>MSPITREERLERRIQDLYANDPQFAAAKPATAITAAIERPGLPLPQIIETVMTGYADRPALAQRSVEFVTDAGTGHTTLRLLPHFETISYGELWDRISALADVLSTEQTVKPGDRVCLLGFNSVDYATIDMTLARLGAVAVPLQTSAAITQLQPIVAETQPTMIAASVDALADATELALSGQTATRVLVFDHHRQVDAHRAAVESARERLAGSAVVETLAEAIARGDVPRGASAGSAPGTDVSDDSLALLIYTSGSTGAPKGAMYPRRNVATFWRKRTWFEGGYEPSITLNFMPMSHVMGRQILYGTLCNGGTAYFVAKSDLSTLFEDLALVRPTELTFVPRVWDMVFDEFQSEVDRRLVDGADR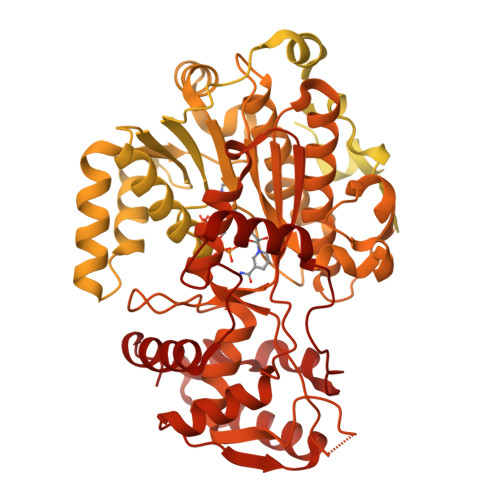VALEAQVKAEIRNDVLGGRYTSALTGSAPISDEMKAWVEELLDMHLVEGYGSTEAGMILIDGAIRRPAVLDYKLVDVPDLGYFLTDRPHPRGELLVKTDSLFPGYYQRAEVTADVFDADGFYRTGDIMAEVGPEQFVYLDRRNNVLKLSQGEFVTVSKLEAVFGDSPLVRQIYIYGNSARAYLLAVIVPTQEALDAVPVEELKARLGDSLQEVAKAAGLQSYEIPRDFIIETTPWTLENGLLTGIRKLARPQLKKHYGELLEQIYTDLAHGQADELRSLRQSGADAPVLVTVCRAAAALLGGSASDVQPDAHFTDLGGDSLSALSFTNLLHEIFDIEVPVGVIVSPANDLQALADYVEAARKPGSSRPTFASVHGASNGQVTEVHAGDLSLDKFIDAATLAEAPRLPAANTQVRTVLLTGATGFLGRYLALEWLERMDLVDGKLICLVRAKSDTEARARLDKTFDSGDPELLAHYRALAGDHLEVLAGDKGEADLGLDRQTWQRLADTVDLIVDPAALVNHVLPYSQLFGPNALGTAELLRLALTSKIKPYSYTSTIGVADQIPPSAFTEDADIRVISATRAVDDSYANGYSNSKWAGEVLLREAHDLCGLPVAVFRCDMILADTTWAGQLNVPDMFTRMILSLAATGIAPGSFYELAADGARQRAHYDGLPVEFIAEAISTLGAQSQDGFHTYHVMNPYDDGIGLDEFVDWLNESGCPIQRIADYGDWLQRFETALRALPDRQRHSSLLPLLHNYRQPERPVRGSIAPTDRFRAAVQEAKIGPDKDIPHVGAPIIVKYVSDLRLLGLL[3x]>MNLTIKEEDFTNTFMKNEESFNTFRVTKVKRWNAKRLFKILFVTVFIVLAGGFSYYIFENFVFQKNRKINHIIKTSKYSTVGFNIENSYDRLMKTIKEHKLKNYIKESVKLFNKGLTKKSYLGSEFDNVELKDLANVLSFGEAKLGDNGQKFNFLFHTASSNVWVPSIKCTSESCESKNHYDSSKSKTYEKDDTPVKLTSKAGTISGIFSKDLVTIGKLSVPYKFIEMTEIVGFEPFYSESDVDGVFGLGWKDLSIGSIDPYIVELKTQNKIEQAVYSIYLPPENKNKGYLTIGGIEERFFDGPLNYEKLNHDLMWQVDLDVHFGNVSSKKANVILDSATSVITVPTEFFNQFVESASVFKVPFLSLYVTTCGNTKLPTLEYRSPNKVYTLEPKQYLEPLENIFSALCMLNIVPIDLEKNT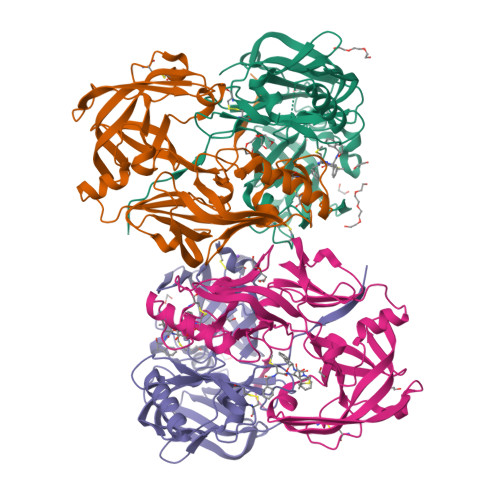FVLGDPFMRKYFTVYDYDNHTVGFALAKNL[4x]>MMKTRGFELITDYTDENLLPKRETAHAAGYDLKVAERTEISAGAIVLVPTGVKAYMQVGEVLYLFDRSSNPRKKGLVLINSVGVIDGDYYNNPNNEGHIFAQMKNMTDQTVVLEAGERVVQGVFMPFLLIDGDKATGTRTGGFGST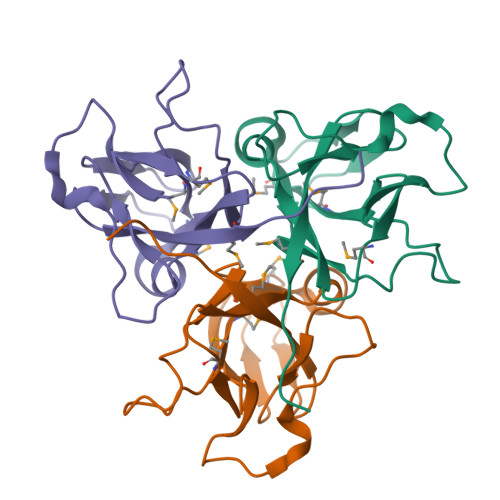GG[3x]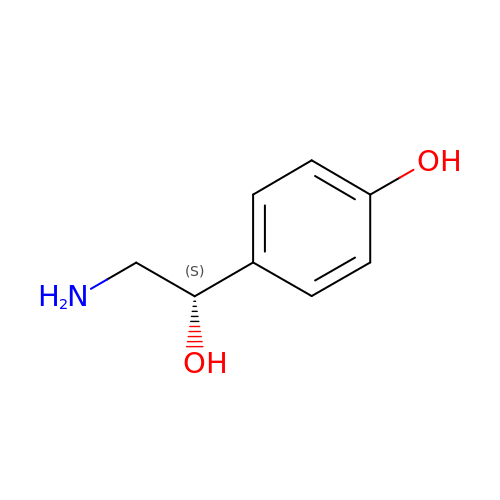4-(2S-AMINO-1-HYDROXYETHYL)PHENOL | C8 H11 N O2 | QHGUCRYDKWKLMG-MRVPVSSYSA-N> MGMSMTILPLELIDKCIGSNLWVIMKSEREFAGTLVGFDDYVNIVLKDVTEYDT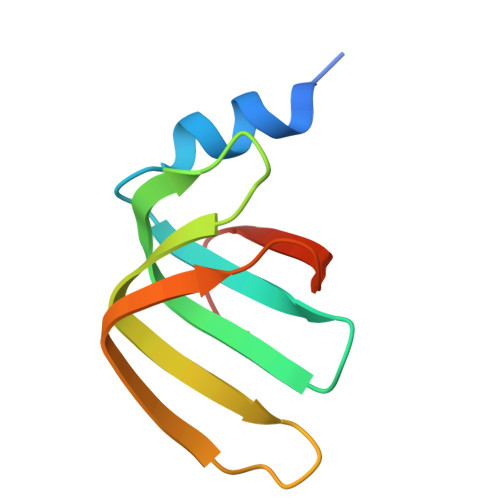VTGVTEKHSEMLLNGNGMCMLIPGGKPE> IVGGKDCPKGECPWQVLLLVNGAQLCGGTLINTIWVVSAAHCFDKIKNWRNLIAVLGEHDLSEHDGDEQSRRVAQVIIPSTYVPGTTNHDIALLRLHQPVVLTDHVVPLCLPERTFSERTLAFVRFSLVSGWGQLLDRGATALVLQVLNVPRLMTQDCLQQSRKVGDSPNITEYMFCAGYSDG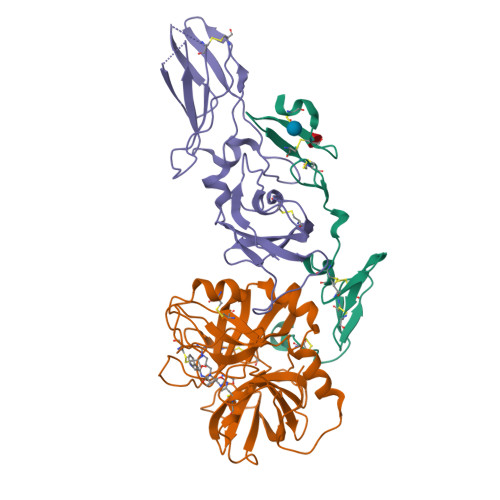SKDSCKGDSGGPHATHYRGTWYLTGIVSWGQGCATVGHFGVYTRVSQYIEWLQKLMRSEPRPGVLLRAPFP;> ANAFLEELRPGSLERECKEEQCSFEEAREIFKDAERTKLFWISYSDGDQCASSPCQNGGSCKDQLQSYICFCLPAFEGRNCETHKDDQLICVNENGGCEQYCSDHTGTKRSCRCHEGYSLLADGVSCTPTVEYPCGKIPILEKRNASKPQGR;> SGTTNTVAAYNLTWKSTNFKTILEWEPKPVNQVYTVQISTKSGDWKSKCFYTTDTECDLTDEIVKDVKQTYLARVFSYPAGNVESTGSAGEPLYENSPEFTPYLETNLGQPTIQSFEQVGTKVNVTVEDERTLVRRNNTFLSLRDVFGKDLIYTLYYWKSSSSGKKTAKTNTNEFLIDVDKGENYCFSVQAVIPSRTVNRKSTDSPVEC> MKLVTVIIKPFKLEDVREALSSIGIQGLTVTEVKGF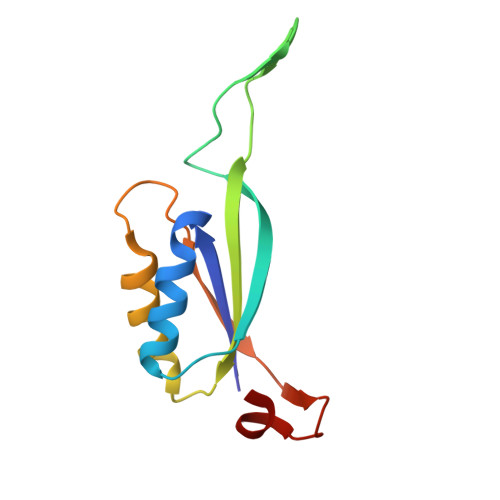GRQKGHAELYRGAEYSVNFLPKVKIDVAIADDQLDEVIDIVSKAAYTGKIGDGKIFVAELQRVIRIRTGEADEAAL> HPETLVKVKDAEDQLGARVGYIELDLNSGKILESFRPEERFPMMSTFKVLLCGAVLSRIDAGQEQLGRRIHYSQNDLVYNSPVTEKHLTDGMTVRELCSAAITMSDNTAANLLLTTIGGPKELTAFLHNMGDHVTRLDRWEPELNEAIPNDERDTTMPAAMATTLRKLLTGELLTLASRQQLIDWMEADKVAGPLLRSALPAGWF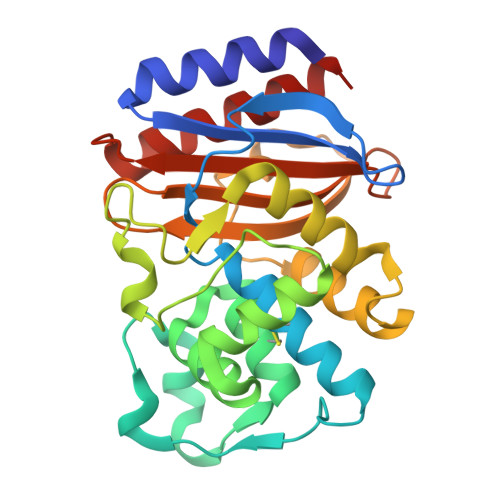IADKSGAGERGSRGIIAALGPDGKPSRIVVIYTTGSQATMDERNRQIAEIGASLIKHW>MLRATVTGNVWSTRRIEGIPAGAFLEVEVEGTGSRMIAFDVLGSGVGEHVLIAQGSVASSWFTGTPPPIDALIIGSIDTRSD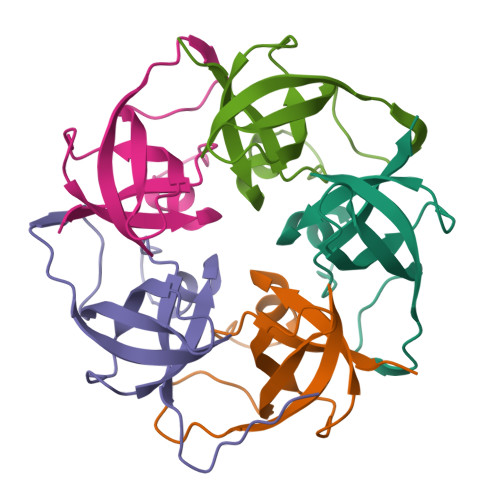SNPAELEHHHHHH[5x]> MSAVKAARYGKDNVRVYKVHKDEKTGVQTVYEMTVCVLLEGEIETSYTKADNSVIVAADSIKNTIYITAKQNPVTPPELFGSILGTHFIEKYNHIHAAHVNIVCHRWTRMDIDGKPHPHSFIRDSEEKRNVQVDVVEGKGIDIKSSLSGLTVLKSTNSQFWGFLRDEYTTLKETWDRILSTDVDATWQWKNFSGLQEVRSHVPKFDATWATAREVTLKTFAEDNSASVQATMYKMAEQILARQQLIETVEYSLPNKHYF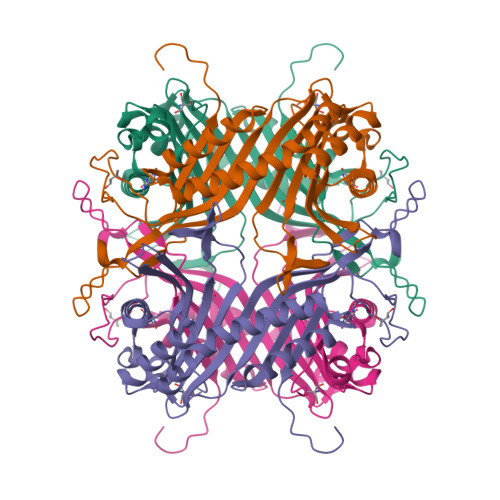EIDLSWHKGLQNTGKNAEVFAPQSDPNGLIKCTVGRSSLKSKL>[6x]MAGFWVGTAPLVAAGRRGRWPPQQLMLSAALRTLKHVLYYSRQCLMVSRNLGSVGYDPNEKTFDKILVANRGEIACRVIRTCKKMGIKTVAIHSDVDASSVHVKMADEAVCVGPAPTSKSYLNMDAIMEAIKKTRAQAV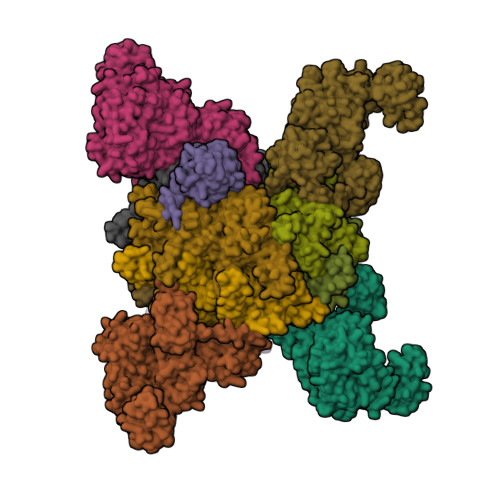HPGYGFLSENKEFARCLAAEDVVFIGPDTHAIQAMGDKIESKLLAKKAEVNTIPGFDGVVKDAEEAVRIAREIGYPVMIKASAGGGGKGMRIAWDDEETRDGFRLSSQEAASSFGDDRLLIEKFIDNPRHIEIQVLGDKHGNALWLNERECSIQRRNQKVVEEAPSIFLDAETRRAMGEQAVALARAVKYSSAGTVEFLVDSKKNFYFLEMNTRLQVEHPVTECITGLDLVQEMIRVAKGYPLRHKQADIRINGWAVECRVYAEDPYKSFGLPSIGRLSQYQEPLHLPGVRVDSGIQPGSDISIYYDPMISKLITYGSDRTEALKRMADALDNYVIRGVTHNIALLREVIINSRFVKGDISTKFLSDVYPDGFKGHMLTKSEKNQLLAIASSLFVAFQLRAQHFQENSRMPVIKPDIANWELSVKLHDKVHTVVASNNGSVFSVEVDGSKLNVTSTWNLASPLLSVSVDGTQRTVQCLSREAGGNMSIQFLGTVYKVNILTRLAAELNKFMLEKVTEDTSSVLRSPMPGVVVAVSVKPGDAVAEGQEICVIEAMKMQNSMTAGKTGTVKSVHCQAGDTVGEGDLLVELE;>[6x]MAAALRVAAVGARLSVLASGLRAAVRSLCSQATSVNERIENKRRTALLGGGQRRIDAQHKRGKLTARERISLLLDPGSFVESDMFVEHRCADFGMAADKNKFPGDSVVTGRGRINGRLVYVFSQDFTVFGGSLSGAHAQKICKIMDQAITVGAPVIGLNDSGGARIQEGVESLAGYADIFLRNVTASGVIPQISLIMGPCAGGAVYSPALTDFTFMVKDTSYLFITGPDVVKSVTNEDVTQEELGGAKTHTTMSGVAHRAFENDVDALCNLRDFFNYLPLSSQDPAPVRECHDPSDRLVPELDTIVPLESTKAYNMVDIIHSVVDEREFFEIMPNYAKNIIVGFARMNGRTVGIVGNQPKVASGCLDINSSVKGARFVRFCDAFNIPLITFVDVPGFLPGTAQEYGGIIRHGAKLLYAFAEATVPKVTVITRKAYGGAYDVMSSKHLCGDTNYAWPTAEIAVMGAKGAVEIIFKGHENVEAAQAEYIEKFANPFPAAVRGFVDDIIQPSSTRARICCDLDVLASKKVQRPWRKHANIPL>[4x]MHHHHHHENLYFQGMQEIIGASLVFLCNEKCEVLEDYGVVFDEKIVEIGDYHNLTLKYPHLKAQFFENSVLLPAFINAHTHFEFSNNKASFDYGSFSGWLGSVLNNGGAILENCQGAIQNAIMAQLKSG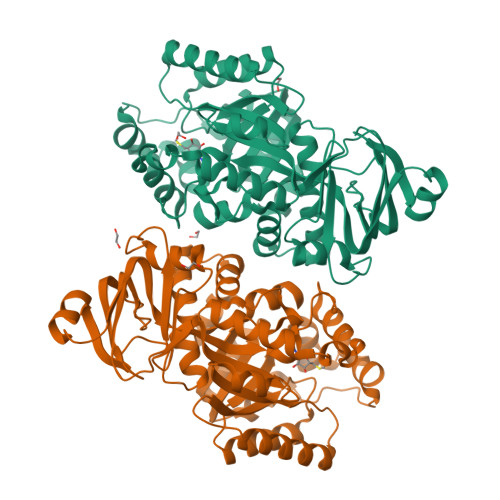VGSVGAISNHLIEVNLLKESPLNAVVFLEFLGSSYSLEKLKAFEAKFKELKDLEDQKLKAALAVHAPYSVQKDMALSVIQLAKDSQSLLSTHFLESLEELEWVENSKGWFENFYQRFLKESNFTSLYEGANDYIDMFKDTHTLFVHNQFASLEALKRIKSQVKNAFLITCPFSNRLLSGKALDLERVREAGLSVSVATDGLSSNISLSLLDELRAFLLSHNMPLLELAKIALLGATRHGAKALALNNGEIETNKRADLSVFGFNEKFTKEQAILQFLLHAKEVERLFLGGKRVI> MKFGNKTKYGKIQEWLRSNNEPDYRMKQITNAIFKQRITRFEDMTNLPKQLREDLINNFGETVLNIKILAEQNSEQVTKVLFEVSDGERVETVIMKYKAGWESFCISSQCGCNFGCKFCATGDIGLKKNLTVDEITDQVLYFHLLGHQIDSISFMGMGEALANRQVFDALDVFTDPNLFALSPRRLSISTIGIIPSIKKLTQEYPQVNLTFSLHSPYSEERSKLMPINDRYPIDEVMNILDEYIRKTSRKVYIAYIMLPGVNDSLEHAKEVVSLLKSRYKSGKLYHVNLIRYNPTISA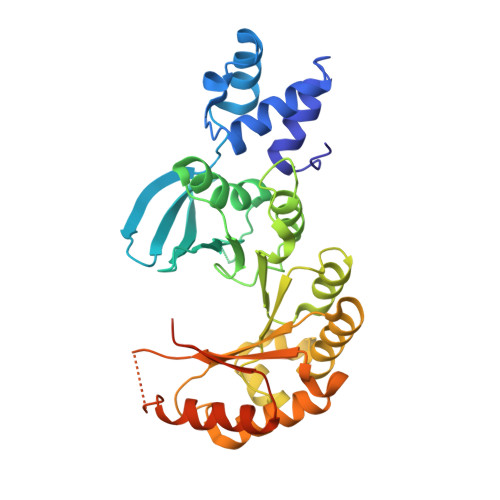PEMYGEANEGQVEAFYKVLKSAGINVTIRSQFGIDIDAACGQLYGNYQNSQ(3R)-1-[(4S)-azepan-4-ylcarbamoyl]-3-(sulfoamino)-L-proline | C12 H22 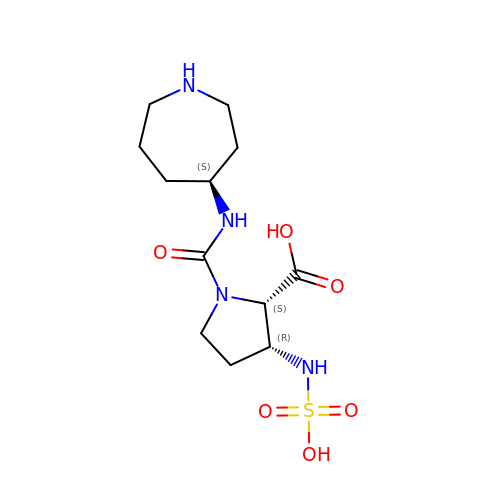N4 O6 S | WWLDRJMXWRULQB-AEJSXWLSSA-N3-MERCAPTO-1-(1,3,4,9-TETRAHYDRO-B-CARBOLIN-2-YL)-PROPAN-1-ONE 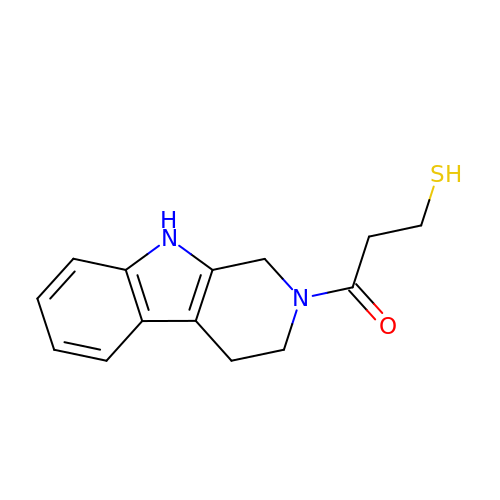| C14 H16 N2 O S | UGWLHSPOMCORRH-UHFFFAOYSA-N2-(3,4-dimethoxyphenoxy)ethyl 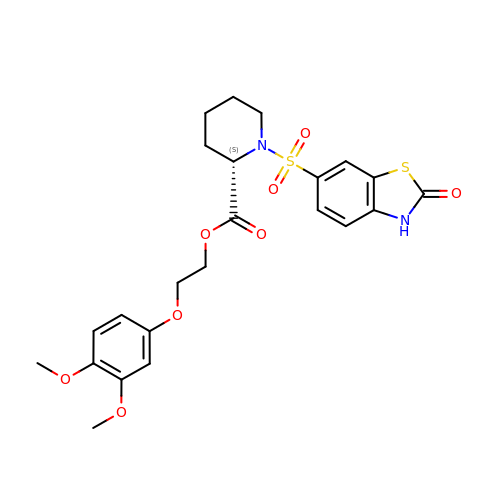(2S)-1-[(2-oxo-2,3-dihydro-1,3-benzothiazol-6-yl)sulfonyl]piperidine-2-carboxylate | C23 H26 N2 O8 S2 | LKFOEMMDLYEDRW-SFHVURJKSA-N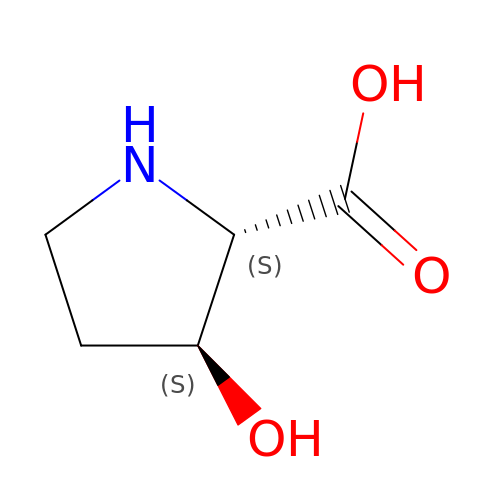3-HYDROXYPROLINE | C5 H9 N O3 | BJBUEDPLEOHJGE-IMJSIDKUSA-N>MRKELVFVLLALFLCAGCNGNKKKMNGEHDLDAANITLDDHTISFYYNWYGNPSVDGEMKHWMHPIALAPGHSGDVGAISGLNDDIACNFYPELGTYSSNDPEIIRKHIRMHIKANVGVLSVTWWGESDYGNQSVSLLLDEAAKVGAKVCFHIEPFNGRSPQTVRENIQYIVDTYGDHPAFYRTHGKPLFFIYDSYLIKPAEWAKLFAAGGEISVRNTKYDGLFIGLTLKESELPDIETACMDGFYTYFAATGFTNASTPANWKSMQQWAKAHNKLFIPSVGPGYIDTRIRPWNGSTTRDRENGKYYDDMYKAAIESGASYISITSFNEWHEGTQIEPAVSKKCDAFEYLDYKPLADDYYLIRTAYWVDEFRKARSAS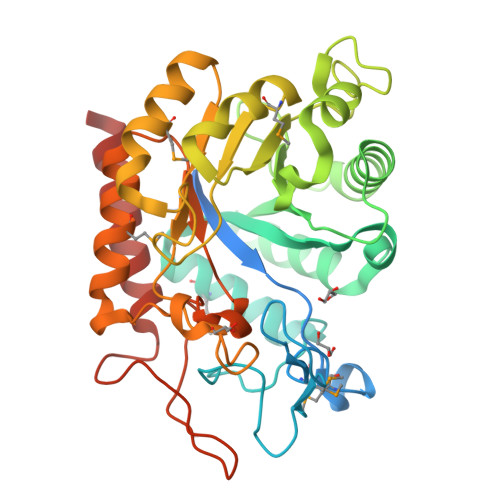EDVQ[2x]> MAIVPFKRDPTFYPSPKMAMKAPPEDLAYVACLYTGTGINRADFIAVVDVNPKSETYSKIVHKVELPYINDELHHFGWNACSSALCPNGKPNIERRFLIVPGLRSSRIYIIDTKPNPREPKIIKVIEPEEVKKVSGYSRLHTVHCGPDAIYISALGNEEGEGPGGILMLDHYSFEPLGKWEIDRGDQYLAYDFWWNLPNEVLVSSEWAVPNTIEDGLKLEHLKDRYGNRIHFWDLRKRKRIHSLTLGEENRMALELRPLHDPTKLMGFINMVVSLKDLSSSIWLWFYEDGKWNAEKVIEIPAEPLEGNLPEILKPFKAVPPLV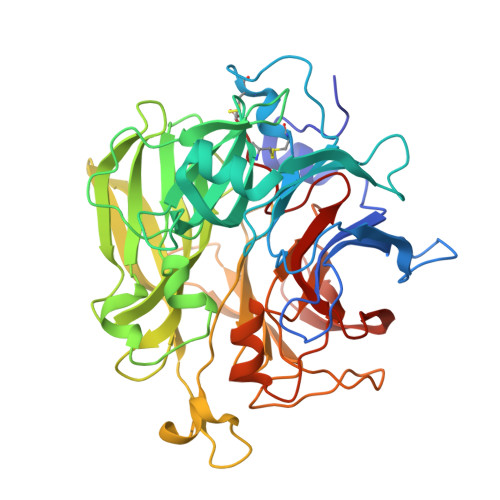TDIDISLDDKFLYLSLWGIGEVRQYDISNPFKPVLTGKVKLGGIFHRADHPAGHKLTGAPQMLEISRDGRRVYVTNSLYSTWDNQFYPEGLKGWMVKLNANPSGGLEIDKEFFVDFGEARSHQVRLSGGDASSDSYCYP> ASPSSELRRALEANEFIPYYQPLSPGQGGRWIGVEVLMRWRHPREGLIRPDLFIPFAERSGLIVPMTRALMRQVAEDLGGHAGKLEPGFHIGFNISATHCHELALVDDCRELLAAFPPGHITLVLELTERELIESSEVTDRLFDELHALGVKIAIDDFGTGHSSLAYLRKFQVDCLKIDQSFVARIGIDTLSGHILDSIVELSAKLDLDIVAEGVETPEQRDYLAARGVDYLQGYLIGRPMPLESLLSSLTVQEGQ;> SPSSELRRALEANEFIPYYQPLSPGQGGRWIGVEVLMRWRHPREGLIRPDLFIPFAERSGLIVPMTRALMRQVAEDLGGHAGKLEPGFHIGFNISATHCHELALVDDCRELLAAFPPGHITLVLELTERELIESSEVTDRLFDELHALGVKIAIDDFGTGHSSLAYLRKFQVDCLKIDQSFVARIGIDTLSGHILDSIVELSAKLDLDIVAEGVETPEQRDYLAARGVDYLQGYLIGRPMPLESLLSSLTVQEG

DGC domains containing the signature GGDEF motif synthesise c-di-GMP from two GTP molecules while EAL1516 and HD-GYP171819 domain-containing PDEs are responsible for the hydrolysis of c-di-GMP to 5′-phosphoguanylyl-(3′-5′)-guanosine (pGpG). Hydrolysis of c-di-GMP by EAL domains has been shown to require the presence of divalent ions, either Mg2+ or Mn2+, with the most efficient reactions occurring at alkaline pH2933. Here we report as yet structurally uncharacterised EAL domains from the core genome of Pseudomonas aeruginosa, PA1727 (MucR) and PA3825.

Ca2+ is a well known inhibitor of EAL-PDE activity. To better understand the reasons for the inhibitory role of Ca2+, we determined PA3825EAL structures in the presence of Mg2+ or Ca2+ ions with bound c-di-GMP. The Mg2+ and Ca2+ complexes show metals in the catalytic centre, annotated as M1 and M2, coordinating the phosphate group of the scissile phosphodiester in c-di-GMP. The Mg2+ and Ca2+ metals in the M1 site superimpose well between the two complexes. In both cases, the metal is coordinated in an octahedral geometry by Glu39, Asn98, Asp130, Asp160, a non-bridging oxygen from the scissile phosphate (P1) of c-di-GMP and a putative in-line attacking water molecule. Significant differences are seen in the positioning of the Asp160 side chain between metal bound complexes, with the second oxygen of Asp160 contacting a peptide nitrogen atom with Mg2+ bound; while the Ca2+ bound complex shows Asp160 bridging between the M1 and M2 metals. The M2 metal shows octahedral coordination for Mg2+ but trigonal bipyramidal coordination geometry for Ca2+. Mg2+ is coordinated by Asp161, Asp183, a non-bridging phosphate (P1) oxygen and two waters. This contrasts with the calcium complex, where Asp183 is not involved in coordination but instead Asp160 and Glu217 make contact to the Ca2+ in the M2 position. The different positioning of Asp160 and different coordination geometry of Ca2+, together with physicochemical properties, thus contribute to the inhibitory effect by calcium4647.>[10x]MTQELGNANFENFIGATEGFSEIAYQFTSHILTLGYAVMLAGLLYFILTIKNVDKKFQMSNILSAVVMVSAFLLLYAQAQNWTSSFTFNEEVGRYFLDPSGDLFNNGYRYLNWLIDVPMLLFQILFVVSLTTSKFSSVRNQFWFSGAMMIITGYIGQFYEVSNLTAFLVWGAISSAFFFHILWVMKKVINEGKEGISPAGQKILSNIWILFLISWTLYPGAYLMPYLTGVDGFLYS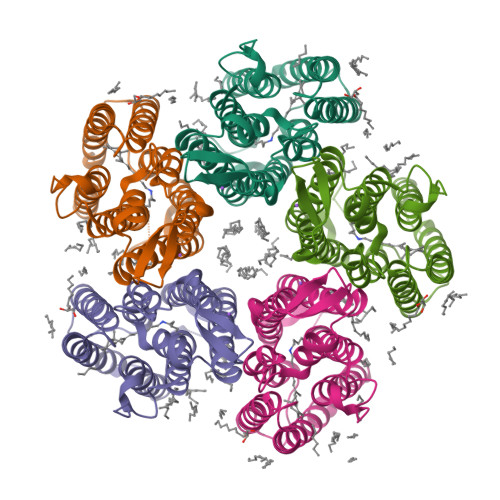EDGVMARQLVYTIADVSSKVIYGVLLGNLAITLSKNKELVEANSLEHHHHHH> SNPTTFSVEAIAAYTPVALIRLLNASGPLQPGHRVDIADARSIYTVGAAASAARARANHNANTIRRTAMFAETDP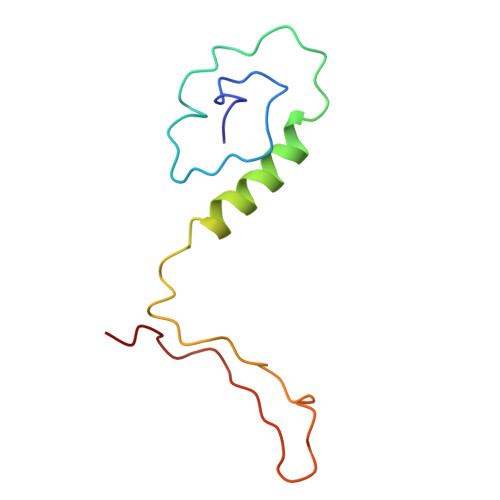MTWLRPTVGLRRTFNPRII> GAMNECAFGT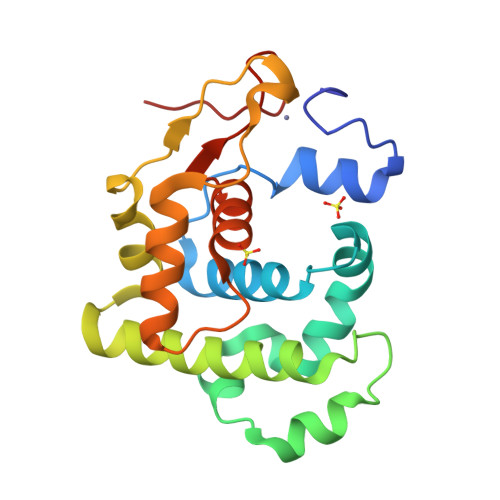KDPVYLNYHDHVWGQPLYDSKALFKLLALQSQHAGLSWLTILKKKEAYEEAFYDFEPEKVAQMTAQDIDRLMTFPNIVHHRKKLEAIVNQAQGYLKIEQAYGSFSKFLWSYVNGKPKDLQYEHASDRITVDDTATQLSKDLKQYGFKFLGPVTVFSFLEAAGLYDAHLKDCPSKPKHN(2S,3aR,5R,6S,7R,7aR)-5-(hydroxymethyl)-2-methyl-2,3a,5,6,7,7a-hexahydro-1H-pyrano[3,2-d][1,3]thiazole-6,7-diol | C8 H15 N O4 S | 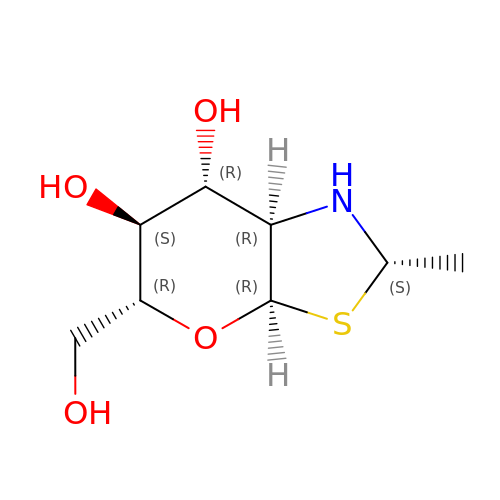XWPUWEBFKDEDIF-GUHFPMLUSA-N>LKKGIIRYLLPAFVLSFTLSTSSQAAPASKPQTPDLEKAEVFGDIDMTTGKQTTVIVELKEKSLAEAKELGKAQTKSKLKSERSKVKKKALKTIKHGKINREYEQVFSGFSMKLPANEIPKLLSDQDVKAVYPNVTYHTDQLKDKDITLSKDAVSPQMDDSAPYIGANDAWKLGYTGKGVKVAIIDTGVEYKHPDLKKNFGQYKGYDFVDNDYDPEETPSGDPRGASTDHGTHVAGTVAANGTIKGVAPDATLLAYRVLGPGGSGTTENVIAGIERAVQDGADVMNLSLGNSVNNPDWATSTALDWAMSEGVTAVTSNGNSGPNNWTVGSPGTSREAISVGATQLPLNEYAVSFGSYSSAKVMGYNKEDDIKALNKKETELIEAGIGEQKDFEGKDLKGKVAVVKRGSIAFVDKADNAKKAGAIGMVVYNNAPGEIEANVPGMSVPTVKLSSEDGEKLVSQLKAGGTKATFHLSVAKSLTEQMADFSSRGPVMDTWMIKPDVSAPGVNIVSTIPTHDPADPYGYGSKQGTSMASPHVAGAAAVIKQAKPKWSPEQIKAALMNTAETLTDADGDVYPHNAQGAGSIRIMKAIKADSLVAPGSYSYGTFMKDKGNETKKETFTIENQSSIRKSYQLEYSFNGTGITVSGTDRVVIPAHQTGKVNAKVKVNAKKVKAGTYEGTVTVREGGKTVAKVPTLLIVKEPDYPRVTSIDVQDGTTQGTYQIETYLPAGAEELAFLVYDSNLDFVGQAGIYKKQDKGYQYFDWNGKVNGDTALPAGEY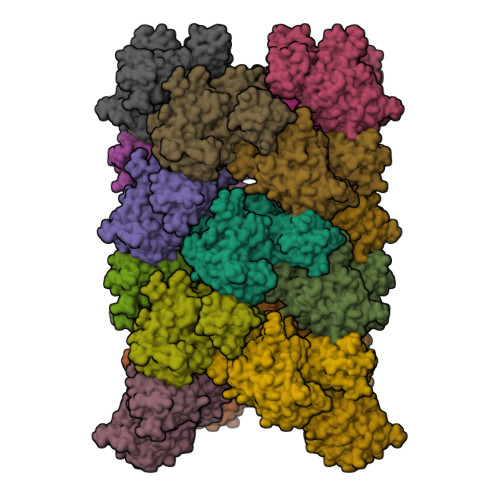YMLAYAANKGKSSQVLTEKPFIIE[18x]>[4x]MAHHHHHHMTPPESVDPDLPEQFRIRQAKRADLLAQGRQPYPVDVPRTHTLLEIRQAYPDLPVDARTGEIVGVTGRVVFARNSGKLCFATLQEGDGTQLQAMISLAEVGQEALDNWKTYVDIGDIVFVHGEVITSKRGELSVLADSWQMAAKALRPLPVAHKEMSEESRVRQRYVDLIVRDQARKVARQRIAVMRAIRSALERRGFLEVETPMLQTLAGGAAARPFVTHSNALDTELYLRIAPELFLKRCLVGGFERVFELNRVFRNEGADSTHSPEFVMLETYQAYGTYDDSAVVTRELIQEVADEAIGTRQVPLPDGTVYDLDGEWESIQMYPSLSEALGEEITPDTPAETLWAIADRLGLDIPRDRGYGHGKLVEELWEHTVGAKLWAPTFVKDFPVETTPLTRSHRSIPGVTEKW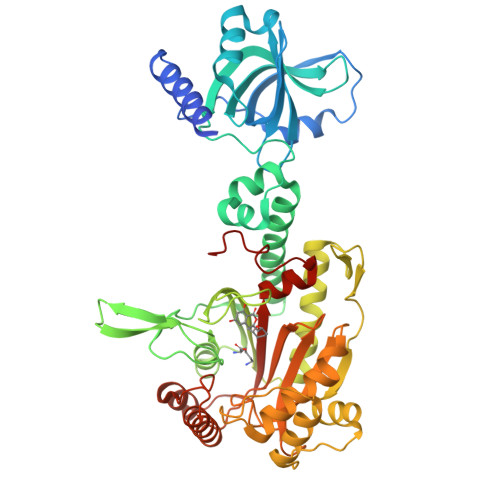DLYVRRIELATGYSELTDPIIQRERFEAQARAAAAGDDEAMALDEDFLAALEYGMPPSTGTGMGIDRLMMTLTGLSIRETVLFPIVKPR> DVAAMDFTDKLIISRPLYISDNADPKCGYCNG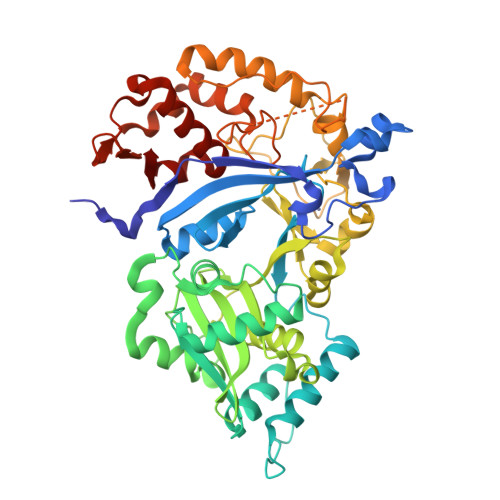KKDSSHKFASPGWSDFYKGDEDKVELQSSTVGFNSELVNAETYDKLCNLGFRRSGSFMYKTDMLRNCCRLYTIRTNEKYLTMSKELKTSLKRFKKKITSPEFKPQPKYVSWIDELCDYEPKSTSFKAVFEPAEFTDEKYDLYVRYQHYIHSDEDNTPSQFESFLCDTPFTDSEITGTEKEWEQLNNWHNLQPGERVTKNGPAHECYYHNGKLIALSVLDFLPSGVSSVYFIWDPDYYDWSLGKVSALRELALVSKIGRPYYYLGYYIDDCPKMNYKAKFGGEILDVCNQKYVPLSKIHQIIKHNELFVGLNSTVASPDSEILITSASDKINFDEPFINAVDDIYGPNGNASQNAITSVAKLRKYGINYSPDLQRSIYKEIPNDGNSTSSASSDKKDVYRIPNVVPGLVPLMEIVSLFESGKMNELNNNVVLFDTKINALRIVRDFISEKPEIKTVITDVIRLIGLDNTKKAIIII>[4x]MKFGIEFVPNEPIQKLCYYVKLAEDNGFEYCWITDHYNNRNVYMALTAIAMNTNKIKLGPGVTNPYVRSPAITASAIATLDELSGGRAVLGIGPGDKATFDALGIEWVKPVTTLKESIEVIRKLLAGERVSYEGKVVKIAGAALAVKPIQKAVPVYMGAQGPKMLETAGMIADGVLINASNPKDFEAAIPLIKKGAEAAGRSMDEIDVAAYACMSVDKNADKAKQAAVPVVAFIAAGSPPVVLERHGIDMEKVEAIRNALKSGNFPEAFKNVDDTMLEAFSIYGTPEDVVEKCKKLAEMGVTQIVAGSPIGPNKETAIKLIGKKVIPALKEALKE

Methylene‐tetrahydropterin reductases catalyze the reduction of a methylene to a methyl group bound to a reduced pterin as C1 carrier in various one‐carbon (C1) metabolisms. F420‐dependent methylene‐tetrahydromethanopterin (methylene‐H4MPT) reductase (Mer) and the flavin‐independent methylene‐tetrahydrofolate (methylene‐H4F) reductase (Mfr) use a ternary complex mechanism for the direct transfer of a hydride from F420H2 and NAD(P)H to the respective methylene group, whereas FAD‐dependent methylene‐H4F reductase (MTHFR) uses FAD as prosthetic group and a ping–pong mechanism to catalyze the reduction of methylene‐H4F. Mutational analysis of four functional amino acids, which are similarly positioned in the three reductase structures, indicated despite the insignificant sequence identity, a common catalytic mechanism with a 5‐iminium cation of methylene‐tetrahydropterin as intermediate protonated by a shared glutamate. Based on mutational and kinetic analysis, evidence has been provided that all three methylene‐tetrahydropterin reductases have the same fold, similar methylene‐tetrahydropterin binding positions, and the same basic catalytic mechanism; however, the binding modes of the C1 carriers and reductants significantly deviate.

For the analysis, Mer from Methanocaldococcus jannaschii was chosen as only the enzyme from this organism can be heterologously and functionally produced thus allowing mutational analyses. For structural comparison with eMTHFR and hMfr, the crystal structures of Mer from M. jannaschii (jMer) with and without F420 were solved. Crystal structures for the apoenzyme of jMer and the binary jMer‐F420 complex were determined at a resolution of 1.8 and 1.9 Å, respectively. The overall structure of jMer is almost identical to those of previously established methanogenic enzymes characterized by a (βα)8‐ or TIM‐barrel fold. The same fold was also found in the structures of MTHFR and Mfr (Gehl et al., 2023; Guenther et al., 1999). The active site of jMer is located in a cleft between the α/β‐barrel domain and a helix‐bundle subdomain composed of five helices. Size‐exclusion chromatography showed that jMer in solution is a homodimer (~80 kDa) as reported in the literature (Miller et al., 2017). The apparent K m and k cat values of jMer are in the range of those of the respective enzymes from methanogenic archaea (M. barkeri, M. marburgensis, and M. kandleri) and sulfate‐reducing archaea (Archaeoglobus fulgidus) (Ma et al., 1991; Ma & Thauer, 1990a; Ma & Thauer, 1990b; Schmitz et al., 1991; te Brommelstroet et al., 1990).> MDKFRVQGPTKLQGEVTISGAKNAALPILFAALLAEEPVEIQNVPKLKDVDTSMKLLSQLGAKVERDGSVHIDARDVNVFCAPYDLVKTMRASIWALGPLVARFGQGQVSLPGGCTIGARPVDLHISGLEQLGATIKLEEGYVKASVDGRLKGAHIVMDKVSVGATVTIMCAATLAEGTTIIENAAREPEIVDTANFLITLGAKISGQGTD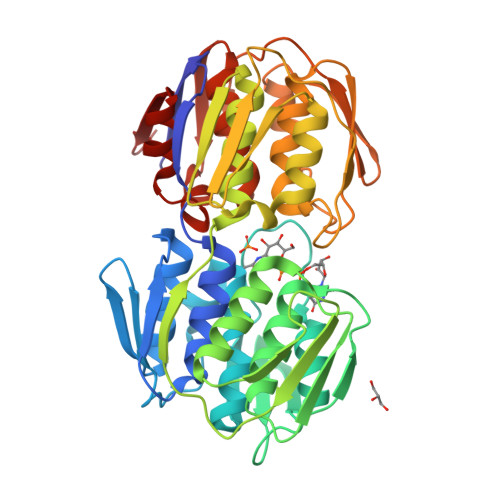RIVIEGVERLGGGVYRVLPDRIETGTFLVAAAISRGKIICRNAQPDTLDAVLAKLRDAGADIEVGEDWISLDMHGKRPKAVNVRTAPHPAFPTDMQAQFTLLNLVAEGTGFITETVFENRFMHVPELSRMGAHAEIESNTVICHGVEKLSGAQVMATDLRASASLVLAGCIAEGTTVVDRIYHIDRGYERIEDKLRALGANIERVKGE>[4x]FETRFEKMDNLLRDPKSEVNSDCLLDGLDALVYDLDFPALRKNKNIDNFLSRYKDTINKIRDLRMKAEDYEVVKVIGRGAFGEVQLVRHKSTRKVYAMKLLSKFEMIKRSDSAFFWEERDIMAFANSPWVVQLFYAFQDDRYLYMVMEYMPGGDLVNLMSNYDVPEKWARFYTAEVVLALDAIHSMGFIHRDVKPDNMLLDKSGHLKLADFGTCMKMNKEGMVRCDTAVGTP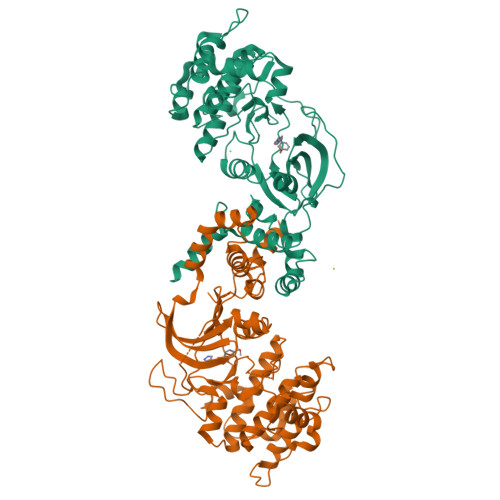DYISPEVLKSQGGDGYYGRECDWWSVGVFLYEMLVGDTPFYADSLVGTYSKIMNHKNSLTFPDDNDISKEAKNLICAFLTDREVRLGRNGVEEIKRHLFFKNDQWAWETLRDTVAPVVPDLSSDIDTSNFDDLEEDKGEEETFPIPKAFVGNQLPFVGFTYYSN>SEPYQIDIRRATNTDAWGPTPKHLAKVLRNRYQVPLYLMTEYTLKRLVDHIATRPKNLYEKARKDYVNYGSEWRVVLKCLVVIEFLLLNVDTGDELNQIRSCLLTHKHILTREIAQFKVKFSNDGKMEIHERGIRKKGELILQYLEDSQFLKKERAKNK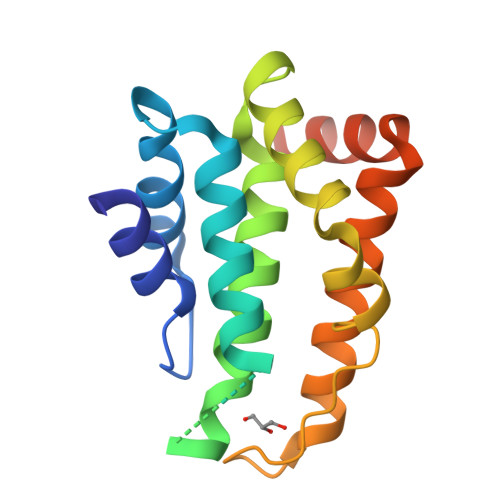KNALEHHHHHH[2x]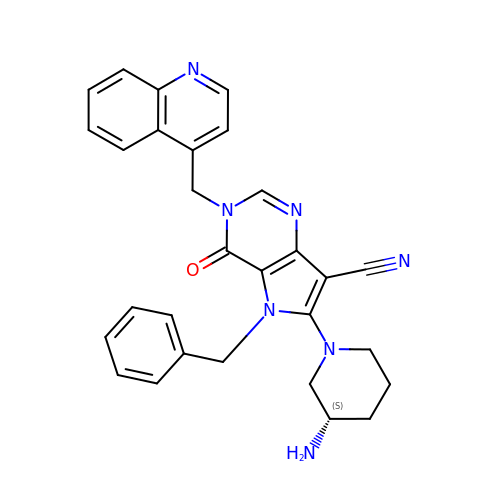6-[(3S)-3-AMINOPIPERIDIN-1-YL]-5-BENZYL-4-OXO-3-(QUINOLIN-4-YLMETHYL)-4,5-DIHYDRO-3H-PYRROLO[3,2-D]PYRIMIDINE-7-CARBONITRILE | C29 H27 N7 O | WRJSBPQWADEDBH-QFIPXVFZSA-N>[7x]MLDSLKSQFQPSFPRLASGHYVHFLMLRHSQSFPVFQTDGVLNTTRTQAGLLEKTDQLSRLVMFKRKQTTPERLAGRELLRNLGLTSADKSAKNLCEYNGEGSCKQCPDCILYGFAIGDSGSERSKVYSDSAFSLGAYEQSHRSFTFNAPFEGGTMSEAGVMRSAINELDHILPEVTFPTVESLRDATYEGFIYVLGNLLRTKRYGAQESRTGTMKNHLVGIVFADGEIFSNLHLTQALYDQMGGELNKPISELCETAATVAQDLLNKEPVRKSELIFGAHLDTLLQEVNDIYQNDAELTKLLGSLYQQTQDYATEFGALSGGKKKAKS;> MTKIYRCKLTLHDNVFFASREMGILYETEKYFHNWALSYAFFKGTIIPHPYGLVGQNAQTPAYLDRDREQNLLHLNDSGIYVFPAQPIHWSYQINTFKAAQSAYYGRSVQFGGKGATKNYPINYGRAKELAVGSEFLTYIVSQKELDLPVWIRLGKWSSKIRVEVEAIAPDQIKTASGVYVCNHPLNPLDCPANQQILLYNRVVMPPSSLFSQSQLQGDYWQIDRNTFLPQGFHYGATTAIAQDSPQLSLLDTN;> MTTLLQTLLIRTLSEQKDYILLEYFQTILPALEEHFGNTSGLGGSFISHQKHFGTQGYDTEKAKKMAQGFAKKGDQTLAAHILNALLTTWNVMQ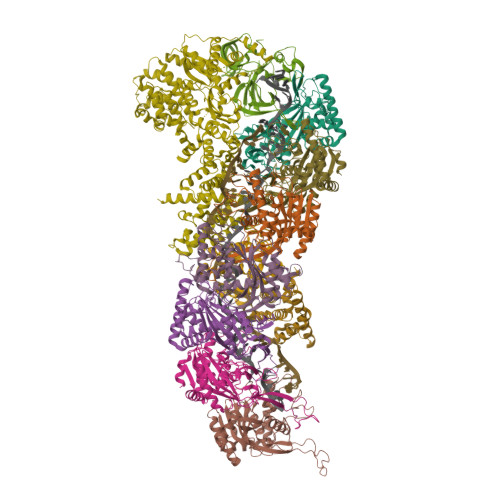ELEFPLNDIERRLLCLGITLHDYDKHCHAQDMAAPEPDNIQEIINICLELGKRLNFDEFWADWRDYIAEISYLAQNTHGKQHTNLISSNWSNAGYPFTIKERKLDHPLRHLLTFGDVAVHLSSPHDLVSSTMGDRLRDLLNRLGIEKRFVYHHLRDTTGILSNAIHNVILRTVQKLDWKPLLFFAQGVIYFAPQDTEIPERNEIKQIVWQGISQELGKKMSAGDVGFKRDGKGLKVSPQTSELLAAADIVRILPQVISVKVNNAKSPATPKRLEKLELGDAEREKLYEVADLRCDRLAELLGLVQKEIFLLPEPFIEWVLKDLELTSVIMPEETQVQSGGVNYGWYRVAAHYVANHATWDLEEFQEFLQGFGDRLATWAEEEGYFAEHQSPTRQIFEDYLDRYLEIQGWESDHQAFIQELENYVNAKTKKSKQPICSLSSGEFPSEDQMDSVVLFKPQQYSNKNPLGGGQIKRGISKIWSLEMLLRQAFWSVPSGKFEDQQPIFIYLYPAYVYAPQVVEAIRELVYGIASVNLWDVRKHWVNNKMDLTSLKSLPWLNEEVEAGTNAQLKYTKEDLPFLATVYTTTREKTDTDAWVKPAFLALLLPYLLGVKAIATRSMVPLYRSDQDFRESIHLDGVAGFWSLLGIPTDLRVEDITPALNKLLAIYTLHLAARSSPPKARWQDLPKTVQEVMTDVLNVFALAEQGLRREKRDRPYESEVTEYWQFAELFSQGNIVMTEKLKLTKRLVEEYRRFYQVELSKKPSTHAILLPLSKALEQILSVPDDWDEEELILQGSGQLQAALDRQEVYTRPIIKDKSVAYETRQLQELEAIQIFMTTCVRDLFGEMCKGDRAILQEQRNRIKSGAEFAYRLLALEAQQNQN;>[2x]MTEKLKLTKRLVEEYRRFYQVELSKKPSTHAILLPLSKALEQILSVPDDWDEEELILQGSGQLQAALDRQEVYTRPIIKDKSVAYETRQLQELEAIQIFMTTCVRDLFGEMCKGDRAILQEQRNRIKSGAEFAYRLLALEAQQNQN> MDETGKE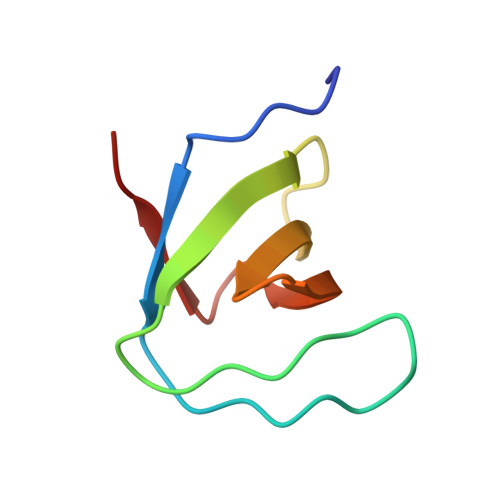LVLALYDYQEKSPREVTMKKGDILTLLNSTNKDWWKVEVNDRQGFVPAGYVKKLD> GMAEYEDRYWTSSDGLRLHFRAYEGDISRPPVLCLPGLTRNARDFEDLATRLAGDWRVLCPEMRGRGDSDYAKDPMTYQPMQYLQDLEALLAQEGIERFVAIGTSLGGLLTMLLAAANPARIAAAVLNDVGPEVSPEGLERIRGYVGQGRNFETWMHAARALQESSGDVY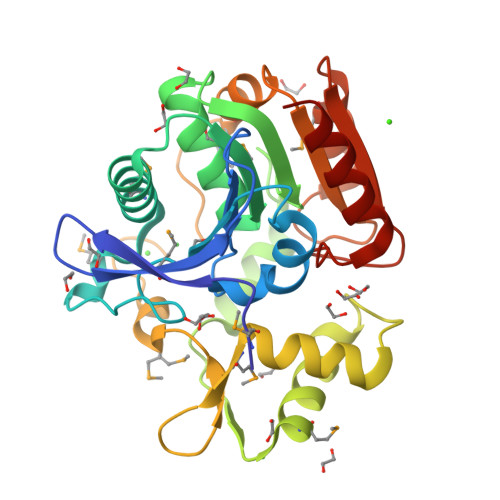PDWDITQWLRYAKRIMVLGSSGRIAFDYDMKIAEPFEAPVGATPQVDMWPLFDALATRPLLVLRGETSDILSAQTAAKMASRPGVELVTLPRIGHAPTLDEPESIAAIGRLLERV> FNDNYSSTSTVYATSNEATDSRGSEHLRYPYLECIKIGMSRDYLENCVKVSFPTSQDMFYDAYPSTESDGAKTRTKEDFSARLLAGDYDSLQKLYIDFYLAQTTFDWEIPTRDQIETLVNYANEGKLSTALNQEYITGRFLTKENGRYDIVNVGGVPDNTPVKLPAIVSKRGLMGTTSVVNAIPNEIYPHIKVYEGTLSRLKPGGAMIAVLEYDVNELSKHGYTNLWDVQFKVLVGVPHAETGVIYDPVYEETVKPYQPSNNLTGKKLYNVSTNDMHNGYKW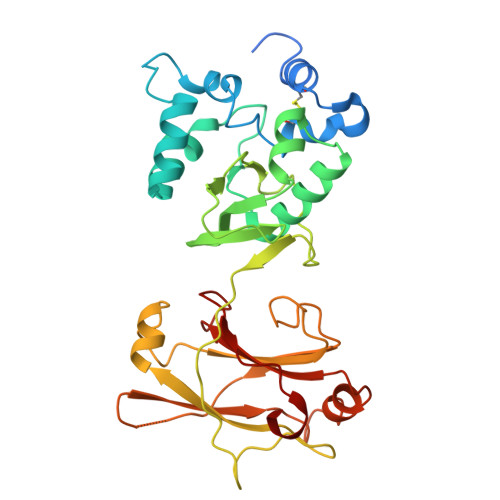SNTMFSNSNYKTQILLTKGDGSGVKLYSKAYSENFK Chitin is a long-chain polymer of β-(1,4)-linked N-acetylglucosamine (GlcNAc) and is synthesized by chitin synthase in the plasma membrane. In this report, we determined seven cryo-electron microscopy (cryo-EM) structures of S. cerevisiae Chs1 in the apo state and in complex with UDP-GlcNAc, UDP-GlcNAc+GlcNAc, UDP, UDP+GlcNAc, PolyB, and NikkoZ. The overall structure of Chs1 reveals a dimer architecture with a twofold symmetry and is ~100 Å tall and 110 Å wide. Each Chs1 monomer is composed of a large cytosolic soluble region and a transmembrane domain (TMD), with both the N-terminus and C-terminus in the cytosol.

Nikkomycin Z (NikkoZ), another peptidyl nucleoside inhibitor of chitin synthase, has shown significant clinical benefits in mammals against pathogenic fungi. The nucleoside moieties of PolyB and NikkoZ are the same 5-aminohexuronic acid N-glycosidically bound to uracil. In contrast, the peptidyl moieties of PolyB contain carbamoylpolyoxamic acid, and NikkoZ contains hydroxypyridylhomothreonine. We determined the structures of Chs1-PolyB and the Chs1-NikkoZ complex at 3.6-Å and 2.4-Å resolution, respectively. Comparison between Chs1 maps in the apo and inhibitor-bound states revealed clearly elongated extra densities corresponding to PolyB and NikkoZ in the active site, consistent with their function as substrate competitive inhibitors. The nucleoside moieties of PolyB and NikkoZ are stabilized by T453, M454, Y455, and K578 at the top of the active site, which are the same residues interacting with the nucleoside group of UDP-GlcNAc. In contrast, unlike the flexible GlcNAc moiety of UDP-GlcNAc extending away from the active site, the peptidyl moieties of PolyB and NikkoZ extend toward the chitin transport channel and form extensive interactions with E457, D602, A677, and W760. Besides, the switch loop of Chs1 is open in our Chs1-PolyB and Chs1-NikkoZ structures. Notably, end part of the peptidyl moieties of PolyB and NikkoZ occupy the GlcNAc acceptor binding site, and thus block the chitin transport channel. Therefore, our structures suggest that the peptidyl nucleoside inhibitors inhibit chitin synthases using a unique mechanism: the nucleoside moiety competes with UDP binding, and the peptidyl moiety induces the switch loop open and blocks the gate of chitin transport channel.

>[2x]MSDQNNRSRNEYHSNRKNEPSYELQNAHSGLFHSSNEELTNRNQRYTNQNASMGSFTPVQSLQFPEQSQQTNMLYNGDDGNNNTINDNERDIYGGFVNHHRQRPPPATAEYNDVFNTNSQQLPSEHQYNNVPSYPLPSINVIQTTPELIHNGSQTMATPIERPFFNENDYYYNNRNSRTSPSIASSSDGYADQEARPILEQPNNNMNSGNIPQYHDQPFGYNNGYHGLQAKDYYDDPEGGYIDQRGDDYQINSYLGRNGEMVDPYDYENSLRHMTPMERREYLHDDSRPVNDGKEELDSVKSGYSHRDLGEYDKDDFSRDDEYDDLNTIDKLQFQANGVPASSSVSSIGSKESDIIVSNDNLTANRALKRSGTEIRKFKLWNGNFVFDSPISKTLLDQYATTTENANTLPNEFKFMRYQAVTCEPNQLAEKNFTVRQLKYLTPRETELMLVVTMYNEDHILLGRTLKGIMDNVKYMVKKKNSSTWGPDAWKKIVVCIISDGRSKINERSLALLSSLGCYQDGFAKDEINEKKVAMHVYEHTTMINITNISESEVSLECNQGTVPIQLLFCLKEQNQKKINSHRWAFEGFAELLRPNIVTLLDAGTMPGKDSIYQLWREFRNPNVGGACGEIRTDLGKRFVKLLNPLVASQNFEYKMSNILDKTTESNFGFITVLPGAFSAYRFEAVRGQPLQKYFYGEIMENEGFHFFSSNMYLAEDRILCFEVVTKKNCNWILKYCRSSYASTDVPERVPEFILQRRRWLNGSFFASVYSFCHFYRVWSSGHNIGRKLLLTVEFFYLFFNTLISWFSLSSFFLVFRILTVSIALAYHSAFNVLSVIFLWLYGICTLSTFILSLGNKPKSTEKFYVLTCVIFAVMMIYMIFCSIFMSVKSFQNILKNDTISFEGLITTEAFRDIVISLGSTYCLYLISSIIYLQPWHMLTSFIQYILLSPSYINVLNIYAFCNVHDLSWGTKGAMANPLGKINTTEDGTFKMEVLVSSSEIQANYDKYLKVLNDFDPKSESRPTEPSYDEKKTGYYANVRSLVIIFWVITNFIIVAVVLETGGIADYIAMKSISTDDTLETAKKAEIPLMTSKASIYFNVILWLVALSALIRFIGCSIYMIVRFFKKVTFR>CACCTAGC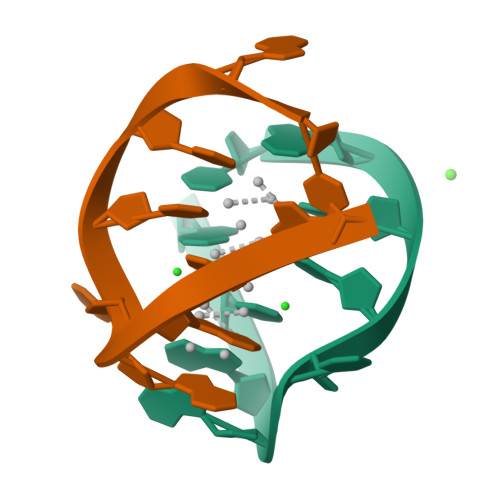G[4x]> MTQLAIGKPAPLGAHYDGQGVNFTLFSAHAERVELCVFDANGQEHRYDLPGHSGDIWHGYLPDARPGLRYGYRVHGPWQPAEGHRFNPAKLLIDPCARQIDGEFKDNPLLHAGHNEPDYRDNAAIAPKCVVVVDHYDWEDDAPPRTPWGSTIIYEAHVKGLTYLHPEIPVEIRGTYKALGHPVMINYLKQLGITALELLPVAQFASEPRLQRMGLSNYWGYNPVAMFALHPAYACSPETALDEFRDA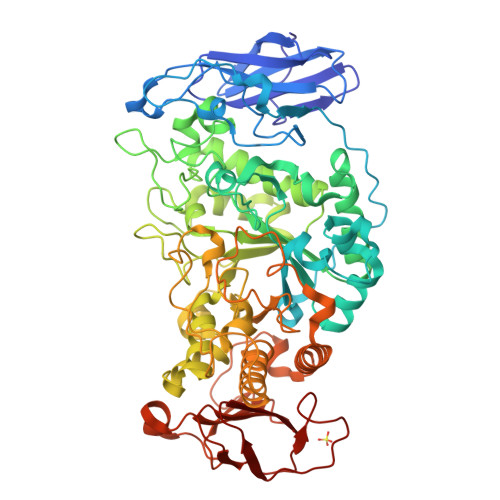IKALHKAGIEVILDIVLNHSAELDLDGPLFSLRGIDNRSYYWIREDGDYHNWTGCGNTLNLSHPAVVDYASACLRYWVETCHVDGFRFDLAAVMGRTPEFRQDAPLFTAIQNCPVLSQVKLIAEPWDIAPGGYQVGNFPPLFAEWNDHFRDAARRFWLHYDLPLGAFAGRFAASSDVFKRNGRLPSAAINLVTAHDGFTLRDCVCFNHKHNEANGEENRDGTNNNYSNNHGKEGLGGSLDLVERRRDSIHALLTTLLLSQGTPMLLAGDEHGHSQHGNNNAYCQDNQLTWLDWSQASSGLTAFTAALIHLRKRIPALVENRWWEEGDGNVRWLNRYAQPLSTDEWQNGPKQLQILLSDRFLIAINATLEVTEIVLPAGEWHAIPPFAGEDNPVITAVWQGPAHGLCVFQR(3S)-1-[(2-fluoroethoxy)acetyl]-N-{[(4P)-4-(6-methylpyridin-3-yl)-1,3-thiazol-2-yl]methyl}piperidine-3-carboxamide | C20 H25 F N4 O3 S | 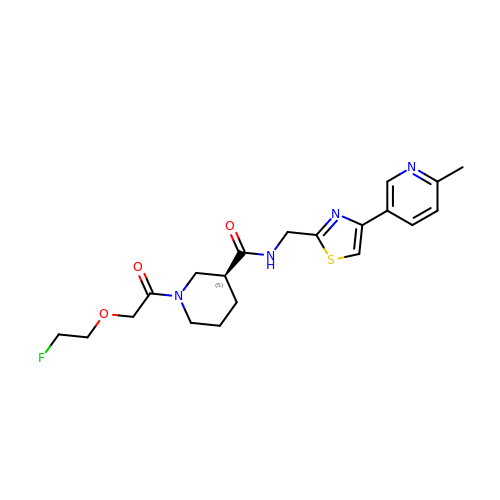BAIMYTMUAKNCDJ-INIZCTEOSA-N>[2x]GPGMATEEMKKLATVMAIGTANPPNCYYQADFPDFYFRVTNSDHLINLKQKFKRLCENSRIEKRYLHVTEEILKENPNIAAYEATSLNVRHK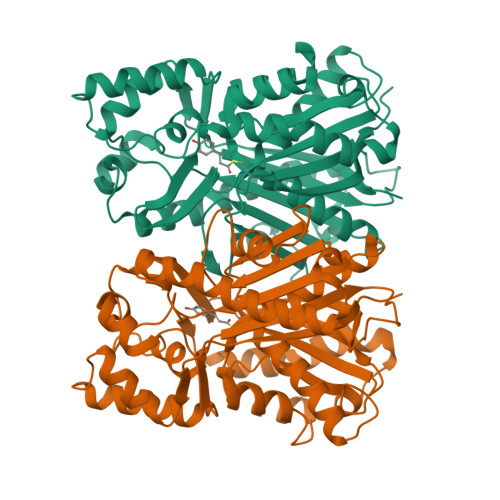MQVKGVAELGKEAALKAIKEWGQPKSKITHLIVCCLAGVDMPGADYQLTKLLDLDPSVKRFMFYHLGCYAGGTVLRLAKDIAENNKGARVLIVCSEMTTTCFRGPSETHLDSMIGQAILGDGAAAVIVGADPDLTVERPIFELVSTAQTIVPESHGAIEGHLLESGLSFHLYKTVPTLISNNIKTCLSDAFTPLNISDWNSLFWIAHPGGPAILDQVTAKVGLEKEKLKVTRQVLKDYGNMSSATVFFIMDEMRKKSLENGQATTGEGLEWGVLFGFGPGITVETVVLRSVPVIS N-(TRANS-4-{(1S,2S)-2-AMINO-3-[(3S)-3-FLUOROPYRROLIDIN-1-YL]-1-METHYL-3-OXOPROPYL}CYCLOHEXYL)-N-METHYLACETAMIDE 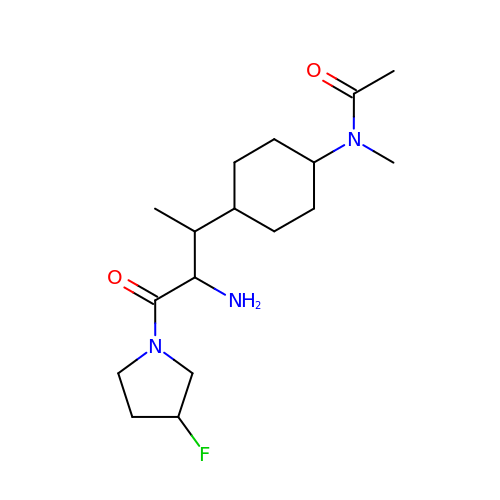| C17 H30 F N3 O2 | BZFQBRSDORUYAB-YDMUCJKGSA-N6-({[(3R,5S)-5-{[(6-amino-4-methylpyridin-2-yl)methoxy]methyl}pyrrolidin-3-yl]oxy}methyl)-4-methylpyridin-2-amine | C19 H27 N5 O2 | 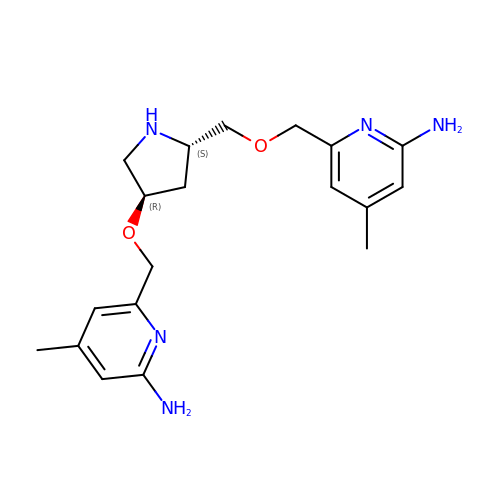NUKSCYDKRQJOFO-WMLDXEAASA-N> ESQPDPMPDDLHKSSEFTGTMGNMKYLYDDHYVSATKVKSVDKFLAHDLIYNISDKKLKNYDKVKTELLNEDLAKKYKDEVVDVYGSNYYVNCYFSSKDNVWWPGKTCMYGGITKHEGNHFDNGNLQNVLVRVYENKRNTISFEVQTDKKSVTAQELDIKARNFLINKKNLYEFNSSPYETGYIKFIENNGNTFWYDMMPAPGDKFDQSKYLMMYNDNKTVDSKSVKIEVH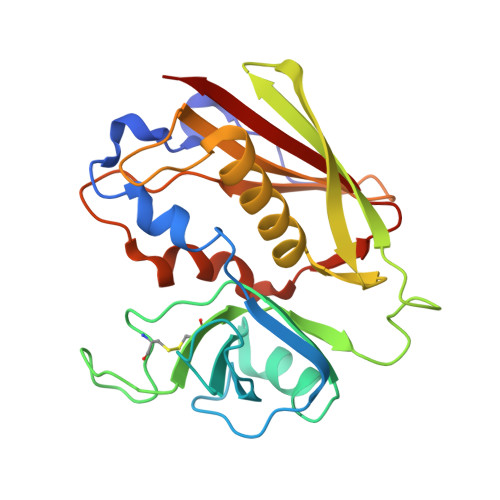LTTKNG>[4x]IIGGRESRPHSRPYMAYLQIQSPAGQSRCGGFLVREDFVLTAAHCWGSNINVTLGAHNIQRRENTQQHITARRAIRHPQYNQRTIQNDIMLLQLSRRVRRNRNVNPVALPRAQEGLRPGTLCTVAGWGRVSMRRGTDTLREVQLRVQRDRQCLRIFGSYDPRRQICVGDRRERK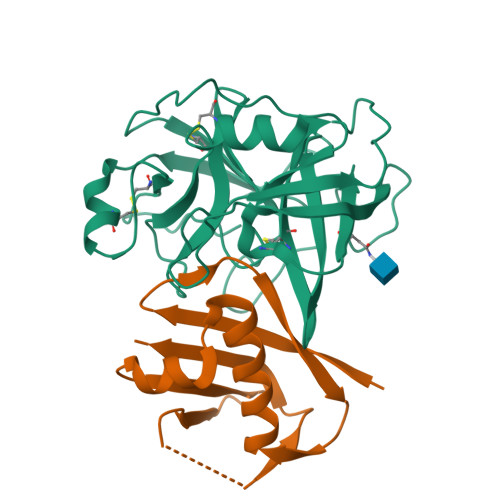AAFKGDSGGPLLCNNVAHGIVSYGKSSGVPPEVFTRVSSFLPWIRTTMR;>GSTIQIPYTITVNGTSQNILSSLTFNKNQNISYKDIENKVKSVLYFNRGISDIDLRLSKQAEYTVHFKNGTKRVIDLKSGIYTADLINTSDIKAISVNVD[4x]> MGNGPPMERAVSSDDIL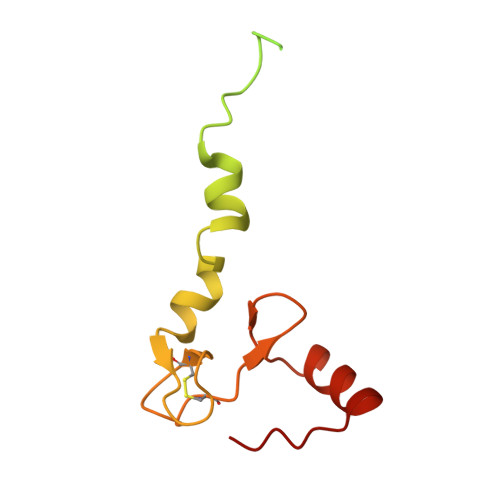TYYNTFIFFIYFNFTNENIYIIYTIYMKVQNTIVYIVLLLIVVVIIWNFTRKEGWSDYNAPNDFMKIYYSNIVEDKKLAEKYPFFGTGPFTGLRCRKPNNVGCNTTWVSGQLVELTPKLKEQIECKFGIQYVKT> SNYLDQMEEYD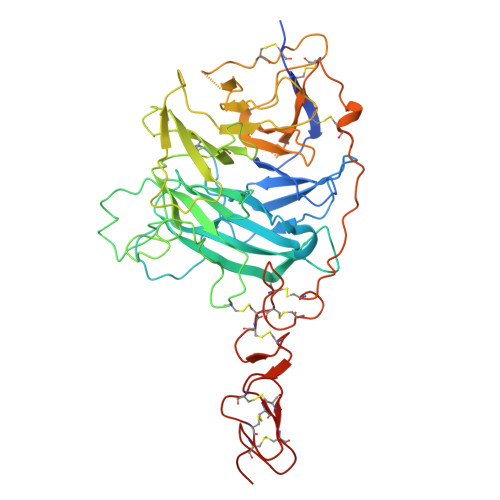KVEEISRKHKHNCFCIQEVVSGLRQPVGALHSGDGSQRLFILEKEGYVKILTPEGEIFKEPYLDIHKLVQSGIKGGDERGLLSLAFHPNYKKNGKLYVSYTTNQERWAIGPHDHILRVVEYTVSRKNPHQVDLRTARVFLEVAELHRKHLGGQLLFGPDGFLYIILGDGMITLDDMEEMDGLSDFTGSVLRLDVDTDMCNVPYSIPRSNPHFNSTNQPPEVFAHGLHDPGRCAVDRHPTDININLTILCSDSNGKNRSSARILQIIKGKDYESEPSLLEFKPFSNGPLVGGFVYRGCQSERLYGSYVFGDRNGNFLTLQQSPVTKQWQEKPLCLGTSGSCRGYFSGHILGFGEDELGEVYILSSSKSMTQTHNGKLYKIVDPKRPLMPEECRATVQPAQTLTSECSRLCRNGYCTPTGKCCCSPGWEGDFCRTAKCEPACRHGGVCVRPNKCLCKKGYLGPQCEHHHHHH>MKLIFLSGVKRSGKDTTADFIMSNYSAVKYQLAGPIKDALAYAWGVFAANTDYPCLTRKEFEGIDYDRETNLNLTKLEVITIMEQAFCYLNGKSPIKGVFVFDDEGKESVNFVAFNKITDVINNIEDQWSVRRLMQALGTDLIVNNFDRMYWVKLFALDYLDKFNSG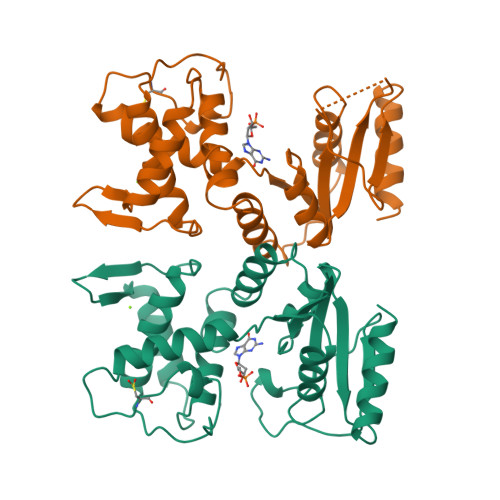YDYYIVPDTRQDHEMDAARAMGATVIHVVRPGQKSNDTHITEAGLPIRDGDLVITNDGSLEELFSKIKNTLKVL[2x]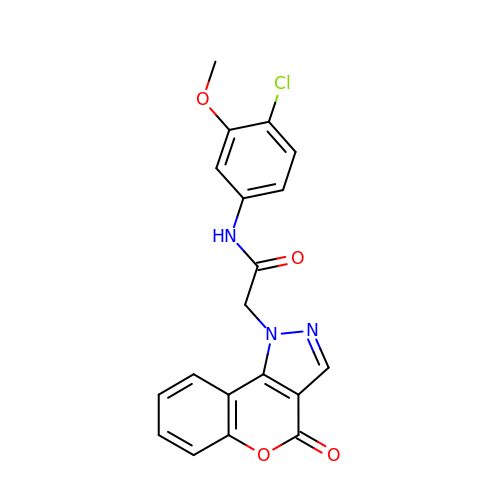N-(4-chloro-3-methoxyphenyl)-2-(4-oxochromeno[4,3-c]pyrazol-1(4H)-yl)acetamide | C19 H14 Cl N3 O4 | DJHSRZJOSYWGCG-UHFFFAOYSA-N5-(AMINOSULFONYL)-4-CHLORO-2-[(2-FURYLMETHYL)AMINO]BENZOIC ACID | C12 H11 Cl N2 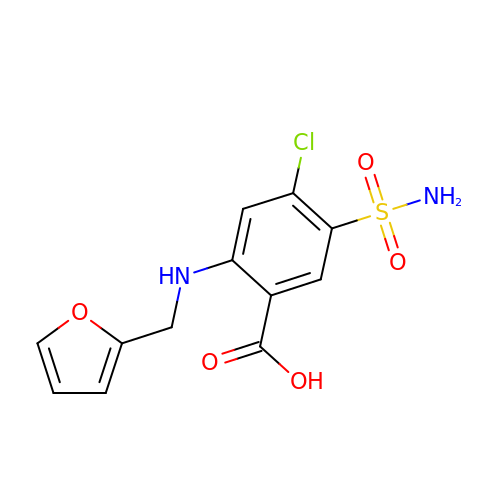O5 S | ZZUFCTLCJUWOSV-UHFFFAOYSA-N>MSSMTTTDNKAFLNELARLVGSSHLLTDPAKTARYRKGFRSGQGDALAVVFPGSLLELWRVLKACVTADKIILMQAANTGLTEGSTPNGNDYDRDVVIISTLRLDKLHVLGKGEQVLAYPGTTLYSLEKALKPLGREPHSVIGSSCIGASVIGGICNNSGGSLVQRGPAYTEMSLFARINEDGKLTLVNHLGIDLGETPEQILSKLDDDRIKDDDVRHDGRHAHDYDYVHRVRDIEADTPARYNADPDRLFESSGCAGKLAVFAVRLDTFEAEKNQQVFYIGTNQPEVLTEIRRHILANFENLPVAGEYMHRDIYDIAEKYGKDTFLMIDKLGTDKMPFFFNLKGRTDAMLEKVKFFRPHFTDRAMQKFGHLFPSHLPPRMKNWRDKYEHHLLLKMAGDGVGEAKSWLVDYFKQAEGDF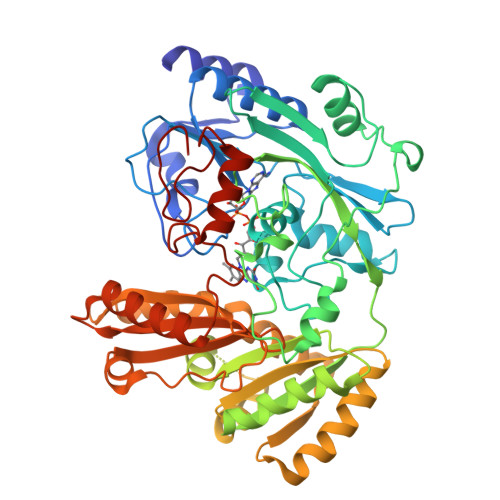FVCTPEEGSKAFLHRFAAAGAAIRYQAVHSDEVEDILALDIALRRNDTEWYEHLPPEIDSQLVHKLYYGHFMCYVFHQDYIVKKGVDVHALKEQMLELLQQRGAQYPAEHNVGHLYKAPETLQKFYRENDPTNSMNPGIGKTSKRKNWQEVE[2x]(2E)-2-METHYLBUT-2-ENEDIOIC ACID 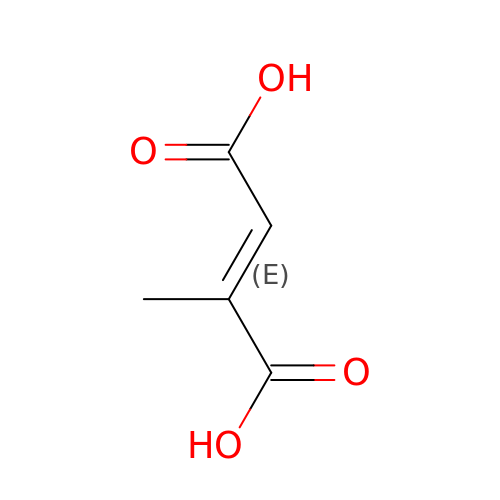| C5 H6 O4 | HNEGQIOMVPPMNR-NSCUHMNNSA-N> LFFLRMWFLYGCCLRFVLFVLCYYMSPRLPSSGNRR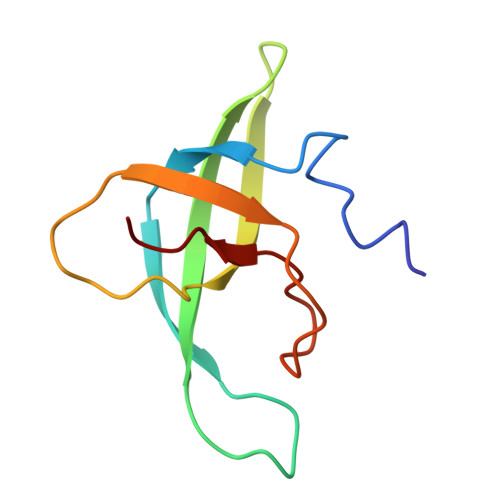VLYAVFYLYNFVWMLRCFFCCFIGLVMSLFIIEGGGFVDLPGVKYYTRIVS> SRGELLLSLCYNPSANSIIVNIIKARNLKAMDIGGTSDPYVKVWLMYKDKRVEKKKTVT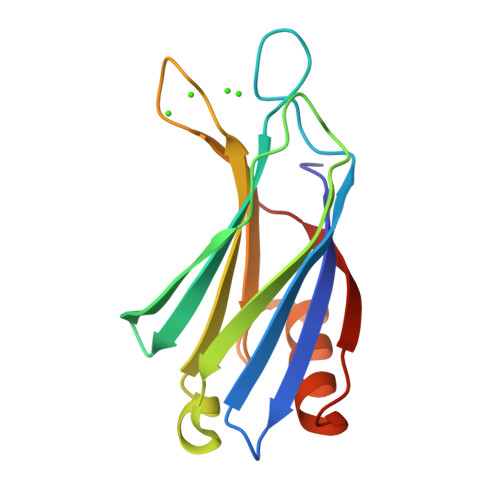KKRNLNPIFNESFAFDIPTEKLRETTIIITVMDKDKLSRNDVIGKIYLSWKSGPGEVKHWKDMIARPRQPVAQWHQLKA> METIGNFIQNMAFPTEN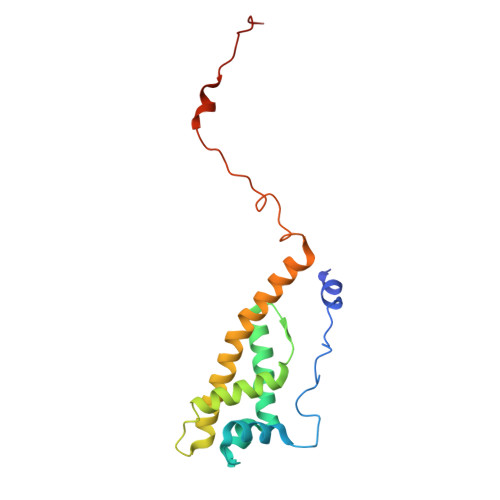PYKLSGDFGNSTLEPTVTAALRILHESPAPFNTEFFSRKNVDFIQKKLISETKRYTSFDIGPQNEDELIMMMAGIYVQDSTFDGNIKAGLRKLNTLVITECLKQILPGVRAYALYVRDASLPFSGGGEEAFKRPELATLKGSKVLSGFLPLDRNAS> MSKPQNNDTLELDDILSQPVKDKERFAAFMMRKLAENKPAQNDNLFGNFKLDFDLDFEVPLIKKSQAKPKSKLPEVQPLGELVSKNSAATEKVNEPPVDQAPNENVPPRRSPTLSPNNRRSMRRSGNVPGSDKLRRHAIRRRSRSCGRQLLPEFEETVNLTRSISSPVNFLPEISSTPCTEKQKEEVAKNTTRVETDKPAEKPMELSQEPEPENPLQTKVTSPARNPILAAEIEQICKERQSSFHKNVLQLDYSGRAPYSRPPTPSSPSVAGLRRTYTMEKGPAPGQLLLSPSHRYDTPSKMPVVKAKRFNQELMVPDTPERQSHDPAWQSEPQPEFVVPETQPQDLGELVQTLSRSAISPIVVINTSNSNRSVRRDAVAMKSVPTSPVTALSSPPIAPSPRRSAAASPQKSIAQLPRVEENMDAIMTDDESDEHPSTVPLNLAPSGGNTTRQRRLRSSNRARATIESQESSMRLLNLHKSVNAKKSKPRKTAIPLNKAPSAPINGEQFARELTRMSNYEILDLRKRNSLNEIYPLNGHRNHRSEKLILEEEIQRELLRRNLMDEAEGLPKQQSSDDSNEDYIPVPPKTQSLRTKSNDRSQGRGRPRSTRRDLPMTTELVNYLGLSQTLETRRKSSKDGKRCLYTKGSSDHEDNDSLSPVKLPRLSKSIQIVPPPPVSLRYSQSLQNLPCSGKFDFDNVVMAAPPDFHDSVNSDAIEIAPPPPEYVVNTRGRSTSGRKSNKNDL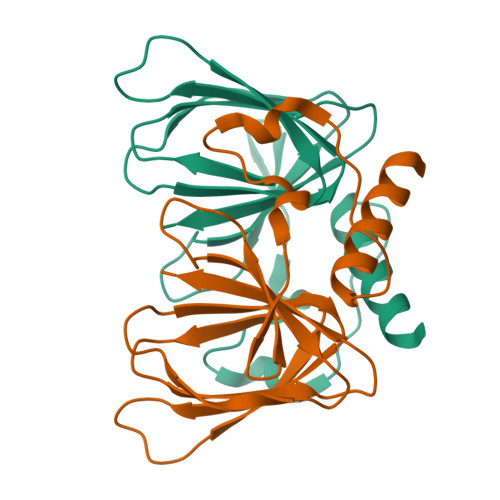VLPPPGYEGGQEEEHDERPSQPRCTAKELQQSTQNGRRAMENELVPPPIEYVEEENRNNEQSRRSTKNGNLVDRNTHNAVEYCEPPEPPEYDDSDHGQASILRRSGKKLQHSKQSVQKSNKEQIIAPSYENNEDYDSDEEPIYNEEYGKEESQNKNVTRRKSDKDEMASHTLECIEGPDPNWNSSCNKQNRNHQNASKSKENDKLANRSSKSQKLSNPRQNAVGTEKSVALSNRGEECTEKSSDVMESLRVNTPTPPIDQNSDDVPSRNPSPSRTLLSDDVPSTSRAALEFLQRSQNMSKSRPPDESSADVVFKKPLAPAPRAKSKKGKSEVDKLKLAKMPVEAEELNTTGIRRSKRGQVPLQMSWCHTMDPSKFNFMSGFIEPRSKNSKTKKGNLSKAKKASATKPKPTVEKNLPDNRGPLCSSTPRISEKLPGAIPHSESLGLSTLTWEETEVQAEAEKVPKKRGRPKKAVGGVQTDTEAEPEPEPEPMISSVAPLTSDQEEPDVPDEQAPYTEAALGPVVFSTPLRDEQEEASTKLMQWLRGVGDAPPSASMSDENASVSSANELIFYQVDGIDYAFYNTKEKAMLGYMRFKPYQKRSMKQAKVHPLKLLVQFGEFNVETLAVGEEKEVHSVLRVGDMIEIDRGTRYSIQNAIDKVSVLMCIRS> IVGGYTCEENSLPYQVSLNSGSHFCGGSLISEQWVVS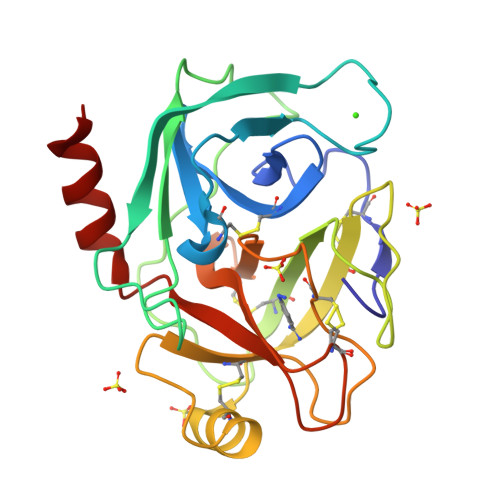AAHCYKTRIQVRLGEHNIKVLEGNEQFINAAKIIRHPKYNRDTLDNDIMLIKLSSPAVINARVSTISLPTAPPAAGTECLISGWGNTLSFGADYPDELKCLDAPVLTQAECKASYPGKITNSMFCVGFLEGGKDSCQRDSGGPVVCNGQLQGVVSWGHGCAWKNRPGVYTKVYNYVDWIKDTIAANS> MEANGLGPQGFPELKNDTFLRAAWGEETDYTPVWCMRQAGRYLPEFRETRAAQDFFSTCRSPEACCELTLQPLRRFPLDAAIIFSDILVVPQALGMEVTMVPGKGPSFPEPLREEQDLERLRDPEVVASELGYVFQAITLTRQRLAGRVPLIGFAGAPWTLMTYMVEGGGSSTMAQAKRWLYQRPQASHQLLRILTDALVPYLVGQVVAGAQALQLFESHAGHLGPQL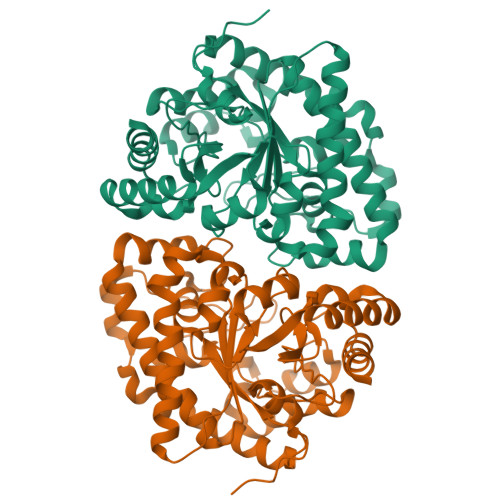FNKFALPYIRDVAKQVKARLREAGLAPVPMIIFAKDGHFALEELAQAGYEVVGLDWTVAPKKARECVGNTVTLQGNLDPCALYASEEEIGQLVKQMLDDFGPHRYIANLGHGLYPDMDPEHVGAFVDAVHKHSRLLRQN Our focus here is on a PLP especially identified as being involved in neurodevelopment, astrotacin-2 (ASTN-2). ASTN-1 and ASTN-2 have been shown to interact directly with each other in vitro in a calcium-independent way with multiple regions of each protein apparently contributing to their interface. Both ASTN-1 and ASTN-2 are integral membrane proteins in which a large C-terminal domain (extracellular for ASTN-1, endosome luminal for ASTN-2) is complemented by an N-terminal cytosolic domain suspended between two transmembrane α-helices. Thus, the endosomal regions of ASTN-2 comprise a smaller N-terminal domain and a larger C-terminal domain whose structure we report here and which we refer to as its endodomain. We describe its unique combination of a canonical MACPF/CDC domain with a minimal epidermal growth factor (EGF)-like repeat (EGF-4), a previously unobserved type of fibronectin type III (Fn(III)) domain in which an additional two β-strands are folded across the core, and an annexin-like domain.

Although most of the crystals diffracted poorly with a high-resolution limit up to 3.6 Å, a native dataset with higher resolution (3.16 Å) was eventually achieved by screening a number of crystals. For crystallization of ASTN2601-1288, 200 nl sitting drops of protein solutions (12 mg ml−1 in 10 mM HEPES pH 7.5, 150 mM NaCl) were mixed with 100 nl of precipitant (12% PEG 20000, 150 mM KSCN, 0.1 M Bis-tris propane pH 7.5–8.5) and equilibrated against 90 µl of crystallization condition. Although we verified that the expressed protein had remained intact such that EGF repeats 2 and 3 (EGF-2 and EGF-3) were present in the crystallized protein, they were not resolved in the structure, presumably due to disorder, though small-angle X-ray scattering (SAXS) data indicate that the domains are folded. The crystal structure contains density consistent with an inositol triphosphate species being bound in a shallow pocket formed by loops from EGF-4 and the β-hairpin slung across the Fn(III) domain. The Fn(III) domain (β12–β15, π1, β16–β19 with the start of β16 and the end of β19 tied together by a disulfide bond) follows directly on from EGF-4 and has the unexpected feature that it is complemented by a 54-residue β-hairpin from the ASTN-2 C-terminus (β20–β21) that folds across the Fn(III) β-sandwich, clasping the edges of both sheets. As such it seems to lock the C-terminus back to the centre of the endodomain, rigidifying the structure. The annexin-like domain is positioned between the Fn(III) domain and the long β-hairpin folded across it (β20–β21) but, functionally, forms the tip of the ASTN-2 endodomain. An annexin-like domain is an unexpected feature of the ASTN-2 structure (α6–α11) which despite undetectable sequence homology with annexin itself superimposes very well on an annexin single repeat (see electronic supplementary material, figure S9 for a superimposition).

>KFNDTLFGEMLHGYNNRTQHVNQGQVFQMTFRENNFIKDFPQLADGLLVIPLPVEEQCRGVLSEPLPDLQLLTGDIRYDEAMGYPMVQQWRVRSNLYRVKLSTITLAAGFTNVLKILTKESSREELLSFIQHYGSHYIAEALYGSELTCIIHFPSKKVQQQLWLQYQKETTELGSKKELKSMPFITYLSGLLTAQMLSDDQLISGVEIRCEEKGRCPSTCHLCRRPGKEQLSPTPVLLEINRVVPLYTLIQDNGTKEAFKSALMSSYWCSGKGDVIDDWCRCDLSAFDANGLPNCSPLLQPVLRLSPTVEPSSTVVSLEWVDVQPAIGTKVSDYILQHKKVDEYTDTDLYTGEFLSFADDLLSGLGTSCVAAGRSHGEVPEVSIYSVIFKCLEPDGLYKFTLYAVDTRGRHSELSTVTLRTACPLVDDNKAEEIADKIYNLYNGYTSGKEQQMAYNTLMEVSASMLFRVQHHYNSHYEKFGDFVWRSEDELGPRKAHLILRRLERVSSHCSSLLRSAYIQSRVETVPYLFCRSEEVRPAGMVWYSILKDTKITCEEKMVSMARNTYGESKGR[4x]>SQNVSLRELAEKLNIYIGFAAINNFWSLSDAEKYMEVARREFNILTPENQMKWDTIHPERDRYNFTPAEKHVEFAEENDMIVHGHTLVWHNQLPGWITGREWTKEELLNVLEDHIKTVVSHFKGRVKIWDVVNEAVSDSGTYRESVWYKTIGPEYIEKAFRWAKEADPDAILIYNDYSIEEINAKSNFVYNMIKELKEKGVPVDGIGFQMHIDYRGLNYDSFRRNLERFAKLGLQIYITEMDVRIPLSGSEEYYLKKQAEVC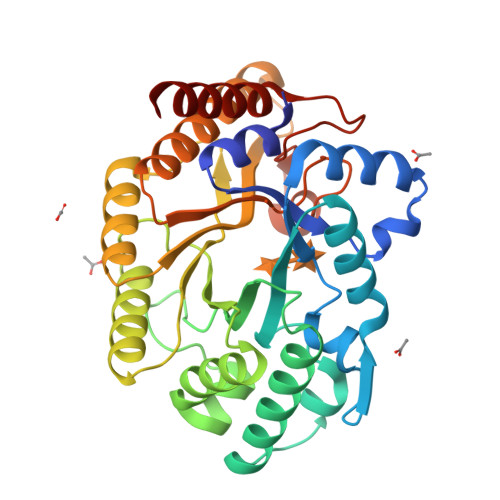AKIFDICLDNPAVKAIQFWGFTDKYSWVPGFFKGYGKALLFDENYNPKPCYYAIKEVLEKKIEERK[2x]>[2x]SMGLVETLRRFRGDVTLDPDTANPELILSEDRRSVQRGDLRQALPDSPERFDPGPCVLGQERFTSGRHYWEVEVGDRTSWALGVCRENVNRKEKGELSAGNGFWILVFLGSYYNSSERALAPLRDPPRRVGIFLDYEAGHLSFYSATDGSLLFIFPEIPFSGTLRPLFSPLSSSPTPMTICRPKGGS

The tripartite motif (TRIM) proteins form one of the largest subfamilies of RING-type E3 ubiquitin ligases, comprising more than 80 members. TRIM family members typically contain a RING domain usually catalyzing ubiquitin transfer; one or two B-box domains mediating protein–protein interactions; and a large coiled-coil domain region, which is involved in self-association or oligomerization with other TRIM E3-ligase proteins (Fiorentini et al., 2020, Ozato et al., 2008). About two-thirds of human TRIM proteins feature a PRYSPRY domain, also known as the B30.2 domain, in their C-terminal region. All characterized family members shared the same overall PRYSPRY twisted β-sandwich fold consisting of a 7-stranded and a 6-stranded antiparallel β-sheet.

A notable exception was the TRIM11 structure, in which a unique subdomain swap was observed. The crystal lattice contained two protein molecules in the asymmetric unit. In chain A, β-strands 7 and 8, usually located at the edge of the concave 6-stranded β-sheet, were displaced and interacted with the corresponding region in chain B, forming a hybrid β-sandwich. The equivalent β-strands in chain B, however, did not interact with chain A but were disordered, resulting in an asymmetrical dimer within the asymmetric unit. These observations raised the question of whether this domain might form a symmetrical subdomain-swapped dimer in solution. However, gel filtration analysis showed that the isolated TRIM11 PRYSPRY domain is largely monomeric in solution. Nevertheless, the observed subdomain swap in the crystal indicates an increased structural plasticity of this region of the TRIM11 PRYSPRY domain that was not seen for other family members. An interesting variation was observed for TRIM11, however, where two β-strands of the 6-stranded β-sheet showed increased structural plasticity, resulting in this segment either being disordered or forming a hybrid sheet with a neighboring molecule. While this assembly is stabilized by crystal packing, it nonetheless reveals the intrinsic flexibility of the swapped β-hairpin motif in this family member.> ECCSRGDAEVVISEWDQVFNAAMAGSSESAIGVAIFDVFFTSSGVSPSMFPGGGDSSSAEFLAQVSRVISGADIAINSLTNRAT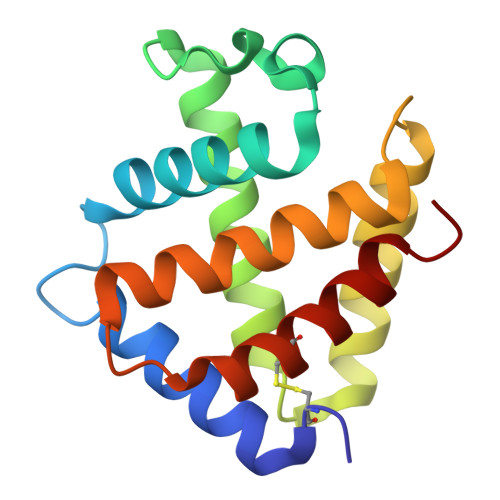CDSLLSHLNAQHKAISGVTGAAVTHLSEAISSVVAQVLPSAHIDAWGYCMAYIAAGIGAGL> MHHHHHH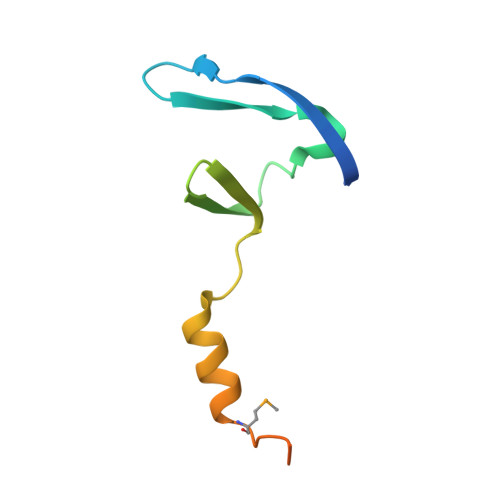ARATGKTFRSGNSEAVRLPRDLAFGADVELTLIRSGDVLTIYPSKGSIADLVATLNQMPRPDSVEIRDEDLFPERPGL>[2x]MAHHHHHHVGTGSNDDDDDKSPSKSSEKRQAVDTAVDGVFIRSLKVNCKVTSRFAHYVVTSQVVNTANEAREVAFDLEIPKTAFISDFAVTADGNAFIGDIKDKVTAWKQYRKAAISGENAGLVRASGRTMEQFTIHLTVNPQSKVTFQLTYEEVLKRNHMQYEIVIKVKPKQLVHHFEIDVDIFEPQGISKLDAQASFLPKELAAQTIKKSFSGKKGHVLFRPTVSQQQSCPTCSTSLLNGHFKVTYDVSRDKICDLLVANNHFAHFFAPQNLTNMNKNVVFVIDISGSMRGQKVKQTKEALLKILGDMQPGDYFDLVLFGTRVQSWKGSLVQASEANLQAAQDFVRGFSLDEATNLNGGLLRGIEILNQVQESLPELSNHASILIMLTDGDP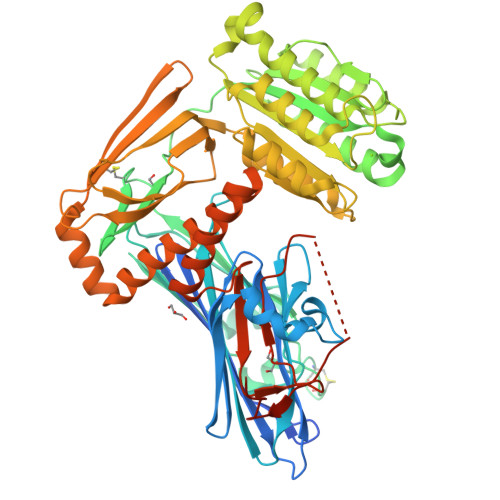TEGVTDRSQILKNVRNAIRGRFPLYNLGFGHNVDFNFLEVMSMENNGRAQRIYEDHDATQQLQGFYSQVAKPLLVDVDLQYPQDAVLALTQNHHKQYYEGSEIVVAGRIADNKQSSFKADVQAHGEGQEFSITCLVDEEEMKKLLRERGHMLENHVERLWAYLTIQELLAKRMKVDREERANLSSQALQMSLDYGFVTPLTSMSIRGMADQDGLKPTIDKPSEDSPPLEMLGPRRTFVLSALQPSPTHSSSNTQRLPDRVTGVDTD> GSTIQ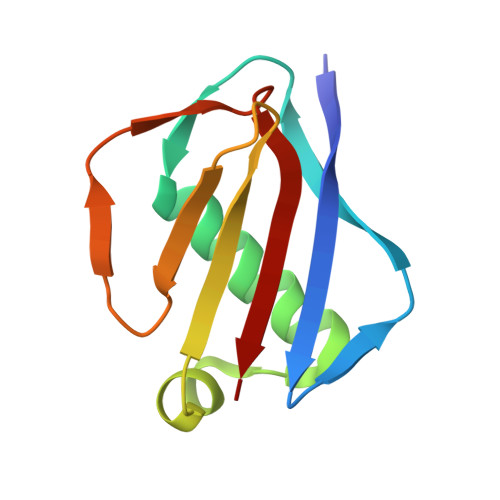IPYTITVNGTSQNILSSLTFNKNQNISYKDIENKVKSVLYFNRGISDIDLRLSKQAEYTVHFKNGTKRVIDLKSGIYTADLINTSDIKAISVNVD Adeno-associated viruses (AAV) are single-stranded DNA packaging viruses of the Parvoviridae and belong to the genus Dependoparvovirus. The virions of the AAVs are composed of non-enveloped capsids with T = 1 icosahedral symmetry and diameters of ≈260 Å. They are assembled from 60 viral proteins (VPs): VP1 (≈82 kDa), VP2 (≈73 kDa), and VP3 (≈61 kDa) in an approximate 1:1:10 ratio. In this study, the structures of the AAV7, AAV11, AAV12, and AAV13 capsids were determined by cryo-EM in an effort to complete the panel of available structures for the defined AAV serotypes.

For AAV11 and AAV12, the closest related AAV serotype is AAV4 based on VP1 or VP3 amino acid sequence ranging from 78 to 81% aa sequence identity. Surprisingly, the structural identity between AAV11 and AAV12 is 98%, which is only surpassed by AAV1 and AAV6 with 99% sequence and structural identity. In contrast, major structural variabilities (vs. AAV2) were seen in VR-I, VR-III, VR-IV, VR-V, VR-VI, VR-VII, and VR-IX for AAV11 and AAV12. Most notably is the 5 aa insertion in VR-V for both AAV11 and AAV12, relative to AAV2, but also to AAV7 and AAV13. In addition, both AAV serotypes possess a single aa insertion in VR-IV and display a different conformation to the other AAV serotypes with the apex of the loop positioned over part of VR-V. This subloop of VR-V and the alternative conformation of VR-IV are responsible for the broader appearance of the 3-fold protrusions of the AAV11 and AAV12 capsids. Similar to previous observations, a structural comparison of empty to the full capsids for the individual AAV serotypes showed them to be largely identical with overall Cα RMSDs ranging from ≈0.2 to 0.3 Å. However, a major difference is the observation of weakly ordered density in the interior of the capsid maps in the full structures interpreted as the packaged genome. This density extends into a pocket underneath the 3-fold symmetry axis and has been interpreted as deoxyadenosine monophosphate (dAMP), which is positioned between conserved prolines 421/632 and histidine 631 (AAV7 numbering). In the AAV serotype structures determined in this study, the histidine side chain preferred the “left” orientation in full capsids. However, in AAV12 and AAV13, weak density was also observed toward the “right” orientation.

>[60x]DGVGNASGDWHCDSTWSEGRVTTTSTRTWVLPTYNNHLYLRIGTTANSNTYNGFSTPWGYFDFNRFHCHFSPRDWQRLINNNWGLRPKSMRVKIFNIQVKEVTTSNGETTVANNLTSTVQIFADSTYELPYVMDAGQEGSFPPFPNDVFMVPQYGYCGVVTGKNQNQTDRNAFYCLEYFPSQMLRTGNNFEVSYQFEKVPFHSMYAHSQSLDRMMNPLLDQYLWHLQSTTTGNSLNQGTATTTYGKITTGDFAYYRKNWLPGACIKQQKFSKNANQNYKIPASGGDALLKYDTHTTLNGRWSNMAPGPPMATAGAGDSDFSNSQLIFAGPNPSGNTTTSSNNLLFTSEEEIATTNPRDTDMFGQIADNNQNATTAPHIANLDAMGIVPGMVWQNRDIYYQGPIWAKVPHTDGHFHPSPLMGGFGLKHPPPQIFIKNTPVPANPNTTFSAARINSFLTQYSTGQVAVQIDWEIQKEHSKRWNPEVQFTSNYGTQNSMLWAPDNAGNYHELRAIGSRFLTHHL>[4x]HHHHHHSMDIEFMAQRAFPNPYADYNKSLAEGYFDAAGRLTPEFSQRLTNKIRELLQQMERGLKSADPRDGTGYTGWAGIAVLYLHLYDVFGDPAYLQLAHGYVKQSLNCLTKRSITFLCGDAGPLAVAAVLYHKMNNEKQAEDCITRLIHLNKIDPHAPNEMLYGRIGYIYALLFVNKNFGVEKIPQSHIQQICETILTSGENLARKRNFTAKSPLMYEWYQEYYVGAAHGL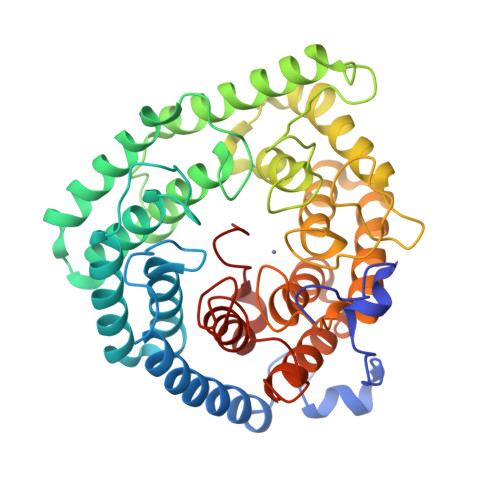AGIYYYLMQPSLQVSQGKLHSLVKPSVDYVCQLKFPSGNYPPCIGDNRDLLVHWCHGAPGVIYMLIQAYKVFREEKYLCDAYQCADVIWQYGLLKKGYGLCHGSAGNAYAFLTLYNLTQDMKYLYRACKFAEWCLEYGEHGCRTPDTPFSLFEGMAGTIYFLADLLVPTKARFPAFEL> MNQPLLSVNNLTHLY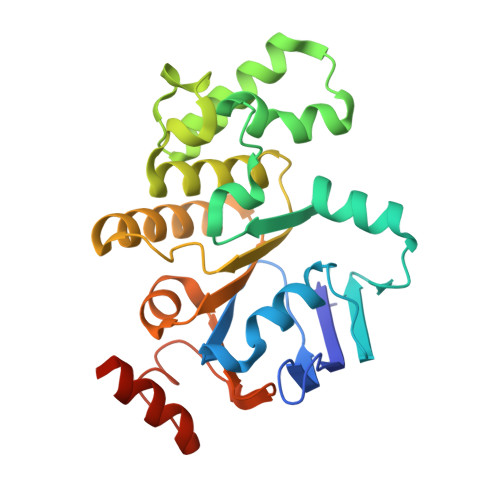APGKGFSDVSFDLWPGEVLGIVGESGSGKTTLLKSISARLTPQQGEIHYENRSLYAMSEADRRRLLRTEWGVVHQHPLDGLRRQVSAGGNIGERLMATGARHYGDIRATAQKWLEEVEIPANRIDDLPTTFSGGMQQRLQIARNLVTHPKLVFMDEPTGGLDVSVQARLLDLLRGLVVELNLAVVIVTHDLGAARLLADRLLVMKQGQVVESGLTDRVLDDPHHPYTQLLVSSVLQNHHHHHH> MGVIKKKRSHHGKASRQQYYSGVQVGGVGSMGAINNNIPSLTSFAEENNYQYGYSGSSAGMNGRSLTYAQQQLNKQRQDFERVRLRPEQLSNIIHDESDTISFRSNLLKNFISSNDAFNMLSLTTVPCDRIEKSRLFSEKTIRYLMQKQHEMKTQAAELQEKPLTPLKYTKLIAAAEDGSRSTKDMIDAVFEQDSHLRYQPDGVVVHRDDPALVGKLRGDLREAPADYWTHAYRDVLAQYHEAKERIRQKEVTAGEAQDEASLQQQQQQDLQQQQQVVTTVASQSPHATATEKEPVPAVVDDP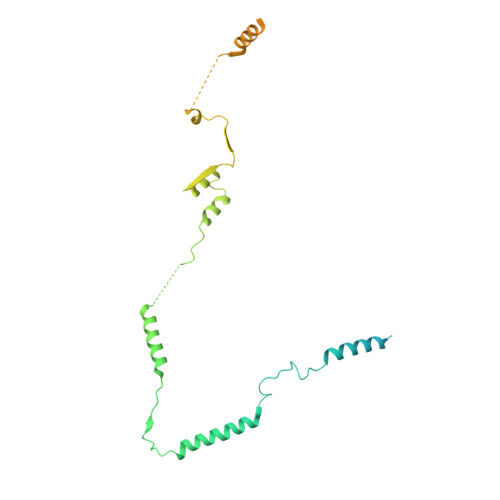LENMFGDYSNEPFNTNFDDEFGDLDAVFF>GPSFWLGNETLKVPLALFALNRQRLCERLRKNPAVQAGSIVVLQGGEETQRYCTDTGVLFRQESFFHWAFGVTEPGCYGVIDVDTGKSTLFVPRLPASHATWMGKIHSKEHFKEKYAVDDVQYVDEIASVLTSQKPSVLLTLRGVNTDSGSVCREASFDGISKFEVNNTILHPEIVECRVFKTDMELEVLRYTNKISSEAHREVMKAVKVGMKEYELESLFEHYCYSRGGMRHSSYTCICGSGENSAVLHYGHAGAPNDRTIQNGDMCLFDMGGEYYCFASDITCSFPANGKFTADQKAVYEAVLRSSRAVMGAMKPGVWWPDMHRLADRIHLEELAHMGILSGSVDAMVQAHLGAVFMPHGLGHFLGIDVHDVGGYPEGVERIDEPGLRSLRTARHLQPGMVLTVEPGIYFIDHLLDEALADPARASFLNREVLQRFRGFGGVRIEEDVVVTDSG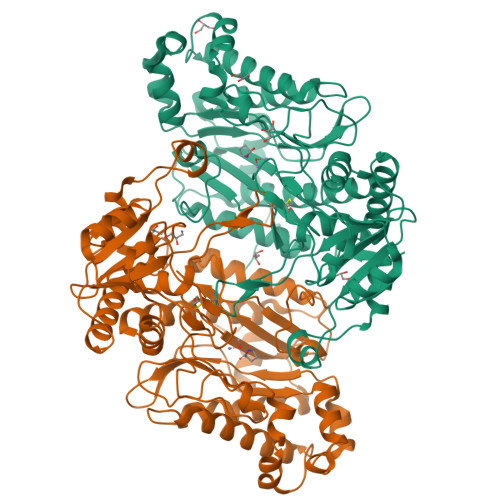IELLTCVPRTVEEIEACMAGCDKAFTPF[2x]>[4x]AENRPVALITMATGYVGPALARTMADRGFDLVLHGTAGDGTMVGVEESFDSQIADLAKRGADVLTISDVDLTTRTGNQSMIERVLERFGRLDSACLVTGLIVTGKFLDMTDDQWAKVKAGNLDMV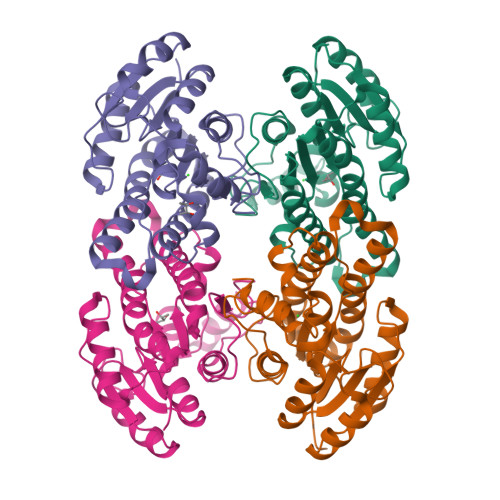FHGLQAVLPPMVAAGAGQCVVFTSATGGRPDPMVSIYGGTRAGANGIVRAVGLEHARHGVQVNAIGTNYMDFPGFLKASRADGDPERRAMIEAQVPLRRLGTMDELSSVTAGLLDGSNRFQTGQFFDFSGGWGA> SNASPTSLEIFATKSSPSGNSARPASVSSRLPGIIFILSSPRSGSTLLRVMLAGHSSLFSPPELHLLPFNTMKERQEQLNLSYLGEGLQKTFMEVKNLDATASQALIKDLESQNLSIQQVYGMLQENIAPRLLVDKSPTYAMEPTILERGEALF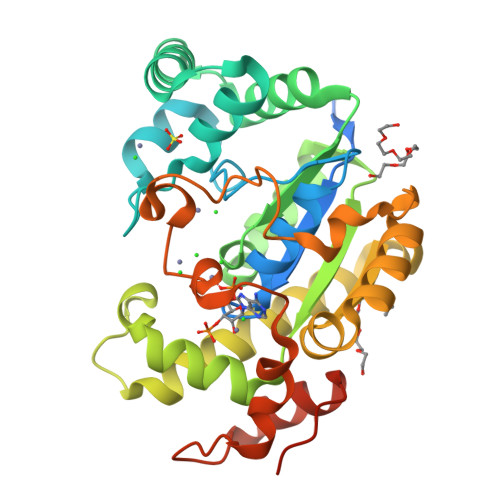ANSKYIYLVRHPYSVIESFVRMRMQKLVGLGEENPYRVAEQVWAKSNQNILNFLSQLEPERQHQIRYEDLVKKPQQVLSQLCDFLNVPFEPELLQPYQGDRMTGGVHAASLSISDPNFLKHNTIDESLADKWKTIQLPYPLKSETQRIASQLSYELPNLVTTPTNQQPQ>AEKNYVMAIDQGTTSSRAIIFDRNGKKIGSSQKEFPQYFPKSGWVEHNANEIWNSVQSVIAGAFIESGIRPEAIAGIGITNQRETTVVWDKTTGQPIANAIVWQSRQSSPIADQLKVDGHTEMIHEKTGLVIDAYFSATKVRWLLDNIEGAQEKADNGELLFGTIDSWLVWKLTDGQVHVTDYSNASRTMLYNIHKLEWDQEILDLLNIPSSMLPEVKSNSEVYGHTRSYAFYGSEVPIAGMAGDQQAALFGQMAFEKGMIKNTYGTGAFIVMNTGEEPQL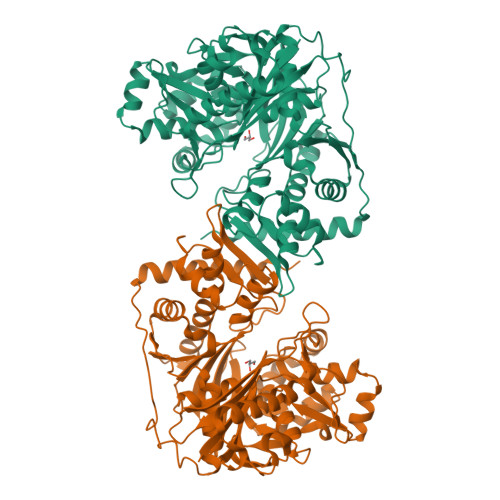SDNDLLTTIGYGINGKVYYALEGSIFVAGSAIQWLRDGLRMIETSPQSEELAAKAKGDNEVYVVPAFTGLGAPYWDSEARGAVFGLTRGTTKEDFVRATLQAVAYQSKDVIDTMKKDSGIDIPLLKVDGGAAKNDLLMQFQADILDIDVQRAANLETTALGAAYLAGLAVGFWKDLDELKSMAEEGQMFTPEMPAEERDNLYEGWKQAVAATQTFKFKAKKEGE[2x]> SMQGPRTRARLGANEVLLVVGGFGSQQSPIDVVEKYDPKTQEWSFLPSITRKRRYVASVS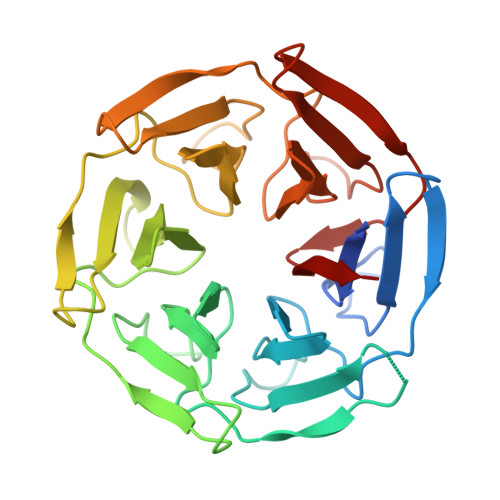LHDRIYVIGGYDGRSRLSSVECLDYTADEDGVWYSVAPMNVRRGLAGATTLGDMIYVSGGFDGSRRHTSMERYDPNIDQWSMLGDMQTAREGAGLVVASGVIYCLGGYDGLNILNSVEKYDPHTGHWTNVTPMATKRSGAGVALLNDHIYVVGGFDGTAHLSSVEAYNIRTDSWTTVTSMTTPRCYVGATVLRGRLYAIAGYDGNSLLSSIECYDPIIDSWEVVTSMGTQRCDAGVCVLRE StARD3 has since been recognized as a carotenoid-binding protein in the primate retina, where its biochemical function of binding lutein with specificity appears to be well suited to recruit this photoprotective molecule. The lutein-binding function of StARD3 resides within the C-terminal START domain comprising residues 216–444, hereafter referred to as StARD3LBD. StARD1 mobilizes cholesterol as the first committed step in steroid biogenesis, and homology between StARD3 and StARD1 suggested that StARD3 also binds cholesterol. The most remarkable structural feature characteristic of StARD3 and StARD1 is a large (∼1000 Å3) solvent-filled cavity.

A crystal structure of the lutein-binding domain of human StARD3 (StAR-related lipid-transfer protein 3; also known as MLN64) has been refined to 1.74 Å resolution. The current and previous structures correspond closely to each other (r.m.s.d. of 0.25 Å), especially in terms of the helix-grip fold constructed around a solvent-filled cavity. The final structural model includes residues 231–444 of StARD3 (the coordinates for residues 216–230 were omitted because no electron density was observed), 224 water molecules, three molecules of ethylene glycol, one sulfate ion and one molecule of l-(+)-tartaric acid. A striking feature of StARD3LBD is the prominent tunnel-like cavity lined by hydrophobic and polar residues with sufficient volume to accommodate a molecule of cholesterol, as demonstrated by modeling. The tunnel-like cavity measures ∼20 Å long from end to end, curves slightly and accommodates 18 solvent molecules, one of which is an ethylene glycol in the current structure. Electron-density maps did not reveal any larger molecules located inside the cavity. The cavity communicates with bulk solvent through two openings, which we will call portal 1 and portal 2. Portal 1 is wider in diameter compared with portal 2 (4  × 8 Å for portal 1 versus 2 × 4 Å for portal 2; distances are measured between solvent-accessible surfaces). A segment of four residues (Gly336, Ala337, Ala338 and Gly339) was associated with weaker-than-average electron density along two alternative chain paths, suggesting that the Ω1 loop is capable of movement just outside portal 1. The new structure includes additional solvent molecules and alternate conformations for several residues, including Arg351, which is located within the cavity, and residues Gly336–Gly339, which are part of the omega loop found just outside the cavity entrance. Structural flexibility in these regions may be necessary for the binding of bulky ligands such as lutein. Modeling experiments indicate that the biologically relevant ligand must protrude from the cavity entrance because it is not possible to completely fit a 30 Å long molecule of lutein into a cavity that measures only 20 Å.

> GSDNESDEEVAGKKSFSAQEREYIRQGKEATAVVDQILAQEENWKFEKNNEYGDTVYTIEVPFHGKTFILKTFLPCPAELVYQEVILQPERMVLWNKTVTACQILQRVEDNTLISYDVSAGAAGGVVSPRDFVNVRRIERRRDRYLSSGIATSHSAKPPTHKYVRGENGPGGFIVLKSASNPRVCTFVWILNTDLKGRLPRYLIHQSLAATMFEFAFHLRQRISELGAR> MAKQYDSVECPFCDEVSKYEKLAKIGQGTFGEVFKARHRKTGQKVALKKVLMENEKEGFPITALREIKILQLLKHENVVNLIEICRTKASPYNRCKGSIYLVFDFCEHDLAGLLSNVLVKFTLSEIKRVMQMLLNGLYYIHRNKILHRDMKAANVLITRDGVLKLADFGLARAFSLAKNSQPNRYTNRVVTLWYRPPELLLGERDYGPPIDLWGAGCIMAEMWTRSPIMQGNTEQHQLALISQLCGSITPEVWPNVDNYELYEKLELVKGQKRKVKDRLKAYVRDPYALDLIDKLLVLDPAQRIDSDDALNHDFFWSDPMPSDLKG;> MEGERKNNNKRWYFTREQLENSPSRRFGVDPDKELSYRQQAANLLQDMGQRLNVSQLTINTAIVYMHRFYMIQSFTRFPGNSVAPAALFLAAKVEGQPKKLEHVIKVAHTCLHPQESLPDTRSEAYLQQVQDLVILESIILQTLGFELTIDHPHTHVVKCTQLVRASKDLAQTSYFMATNSLHLTTFSLQYTPPVVACVCIHLACKWSNWEIPVSTDGKHWWE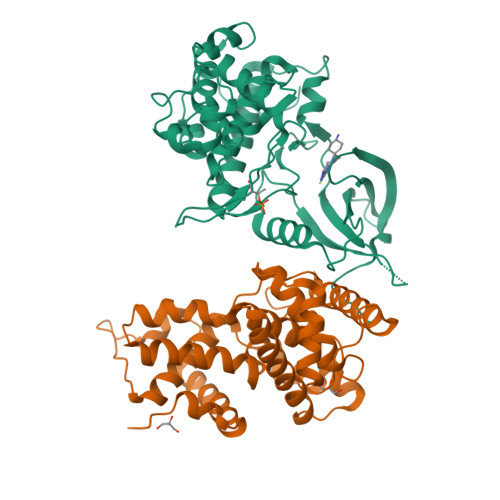YVDATVTLELLDELTHELLQILEKTPNRLKRIWNWRACEAAKKTKADDRGTDEKTSEQTILNMISQSSSDTTIAGLMSMSTSTTSAVPSLPVSEESSSNLTSVEMLPGKRWLSSQPSFKLEPTQGHRTSENLALTGVDHSLPQDGSNAFISQKQNSKSVPSAKVSLKEYRAKHAEELAAQKRQLENMEANVKSQYAYAAQNLLSHHDSHSSVILKMPIEGSENPERPFLEKADKTALKMRIPVAGGDKAASSKPEEIKMRIKVHAAADKHNSVEDSVTKSREHKEKHKTHPSNHHHHHNHHSHKHSHSQLPVGTGNKRPGDPKHSSQTSNLAHKTYSLSSSFSSSSSTRKRGPSEETGGAVFDHPAKIAKSTKSSSLNFSFPSLPTMGQMPGHSSDTSGLSFSQPSCKTRVPHSKLDKGPTGANGHNTTQTIDYQDTVNMLHSLLSAQGVQPTQPTAFEFVRPYSDYLNPRSGGISSRSGNTDKPRPPPLPSEPPPPLPPLPK> MGSDKIHHHHHHENLYFQGMHIHILGICGTFMGSLALLARALGHTV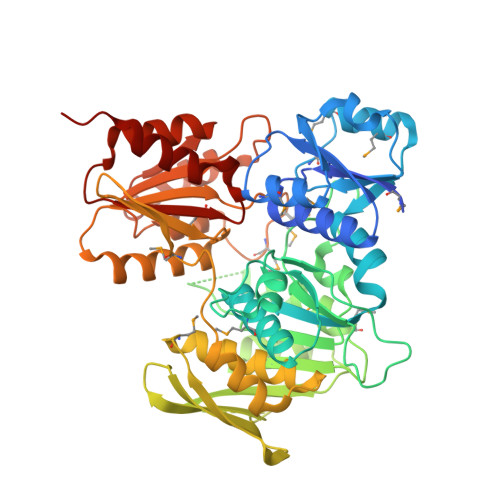TGSDANIYPPMSTQLEQAGVTIEEGYLIAHLQPAPDLVVVGNAMKRGMDVIEYMLDTGLRYTSGPQFLSEQVLQSRHVIAVAGTHGKTTTTTMLAWILHYAGIDAGFLIGGVPLVNTTDTNLQQVFAHSSYLGTEKDDSDNSVNTGYFVIEADEYDSAFFDKRSKFVHYRPRTAILNNLEFDHADIFADLDAIQTQFHHMVRMIPSTGKIIMPAATISLEDTLAKGVWTPIWRTSVIDSTISSVRREDSPLENSQAENSSDWQAELISADGSQFTVSFNDNKEATALVNWSMSGLHNVNNALVAIAAAYNIGVSVKTACAALSAFAGIKRRMELIGDVNDILVFDDFAHHPTAITTTLDGAKKKLADRRLWAIIEPRSNTMKMGIHQDSLAQSATLADHTLWYEPTGLEWGLKEVIDNATIANPSIGSQQVLSSVDDIIKHICTHAKAGDAIVIMSNGGFEGIHQRLLTALGNIVAIL> AGHHHHHHEETLLNTKLETADLKWVTFPQVDGQWEELSGLDEEQHSVRTYEVCDVQRAPGQAHWLRTGWVPRRGAVHVYATLRFTMLECLSLPRAGRSCKETFTVFYYESDADTATALTPAWMENPYIKVDTVAAEHLTRKRPGAEATGKVNVKTLRLGPLSKAGFYLAFQDQGACMALLSLHLFYKK;> IVLEPIYWNSSNSKFLPGQGLVLYPQIGDKLDIICPKVDSKTVGQYEYYKVYMVDKDQADRCTIKKENTPLLNCARPD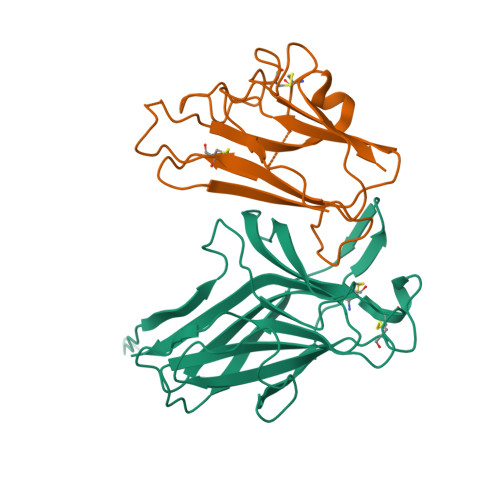QDVKFTIKFQEFSPNLWGLEFQKNKDYYIISTSNGSLEGLDNQEGGVCQTRAMKILMKVG> GSHMASMTGGQQMGRGSMGNLMISFLKKDTQSITLEELAKIIKKCKHVVALTGSGTSAESNIPSFRGSSNSIWSKYDPRIYGTIWGFWKYPEKIWEVIRDISSDYEIEINNGHVAL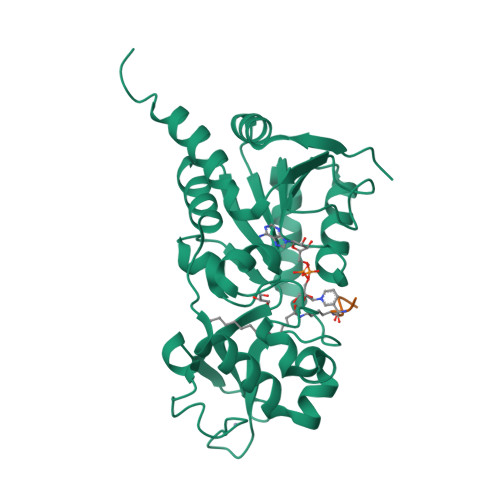STLESLGYLKSVVTQNVDGLHEASGNTKVISLHGNVFEAVCCTCNKIVKLNKIMLQKTSHFMHQLPPECPCGGIFKPNIILFGEVVSSDLLKEAEEEIAKCDLLLVIGTSSTVSTATNLCHFACKKKKKIVEINISKTYITNKMSDYHVCAKFSELTKVANILKGSSEKNKKIM;> KQTARXSTGGWW> MSKLEELDIVSNNILILKKFYTNDEWKNKLDSLIDRIIKAKKIFIFGVGRSGYIGRCFAMRLMHLGFKSYFVGETTTPSYEKDDLLILISGSGRTESVLTVAKKAKNINNNIIAIVCECGNVVEFADLTIPLEVKKSKYLPMGTTFEETALIFLDL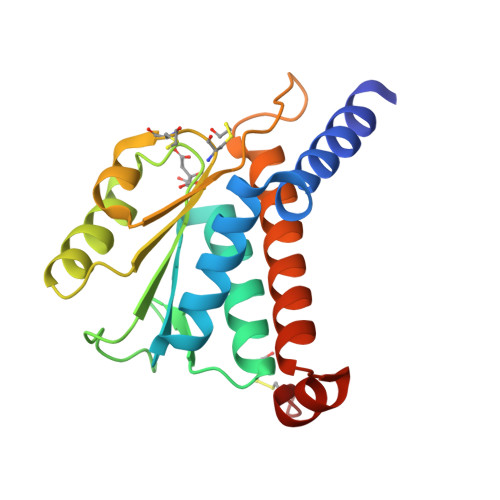VIAEIMKRLNLDESEIIKRHCNLL>GSMKGSRIELGDVTPHNIKQLKRLNQVIFPVSYNDKFYKDVLEVGELAKLAYFNDIAVGAVCCRVDHSQNQKRLYIMTLGCLAPYRRLGIGTKMLNHVLNICEKDGTFDNIYLHVQISNESAIDFYRKFGFEIIETKKNYYKRIEPA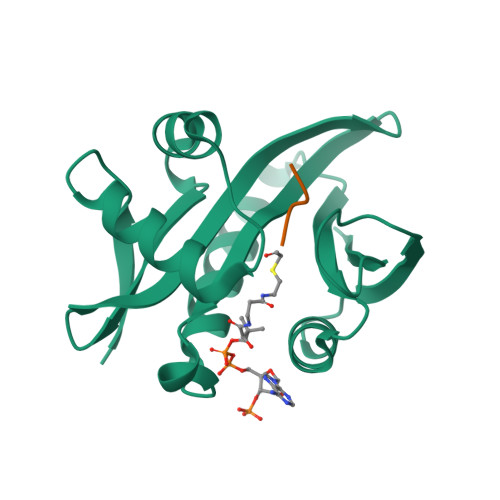DAHVLQKNLKVPSGQNADVQKTDN[6x]> SLVDIFAKALGNCVSASDDALEREVRKFINQYGRVETIAAALAVACGQGSDLRTGTGRGMDRNTENLARAAFIEYGGQPRLAESDGKQSV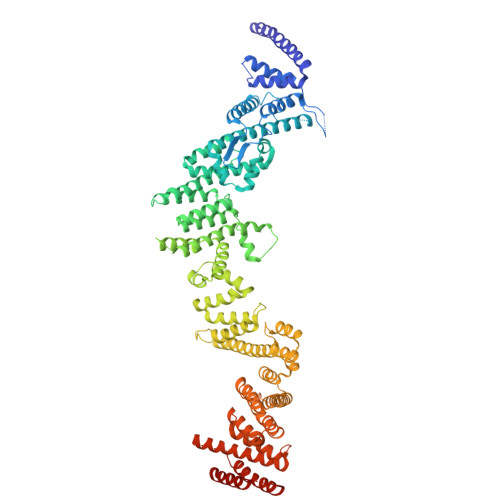SESVRLSSRHDALALYLTRLVRTLWKAKVVQVGSGSDISSTIPTSKLVTIQENVERLRNFLEANKSTIQGLAPPSERLFGRQEDIANQKEHQALHALQKLMESISEGISFVLMLFDERVSDIYARLDAVSQQQLKDLTYEQLFSQTPGKELAKVLVKAIVNRNIASGANVETVADALRRRCGSFCSPDDVVTFKAQEQLQRASEQAHNSPVLRALLAESLRLFEQVAGSLTPANLTTAVEQYISLKYYAGAIQLCLTVAQQKDRGNTALSWVNDGKPANDSRKKAFDERKICYNLIHQVLDKLESDFAGEPELVDGRPTLAATKRMEAYNVVNDSSDEVFHFDLYEWYIEKGWTDRILSIDSPHVITYLQRLAETDFRHAELLCRFYTTRSRFFEAAQVQTNLAKSDLNISLKDRIILLSRAKGNASVNTIGISRQQQQQLNHEASELLEIAHIQDDLLERLVADPRIPEERKAEIEEFLDGPIRTLTDLFNDYADQANYYDLCLLIFHAADFHNPRTILDTWNNLINQSHFEAEQRREYWEIVQAGGDLPAGVIAPIAEPPLPYVYVSQQIQLIAHRTSLDSLIFPVNSLLPVVCAYAINNGQDASIGADPCWPIQLFLNLGVPHALVVQVLENVLDTQEAPFTGRRRKLVVQWIAMAVDMWVREVERRGAMAAAAASGASGSEAVMGSWVSELLGRADQVLTQIAGTGATLRGGAASDAEEIASLRRTVKGLKRSVDM>CTAGGGC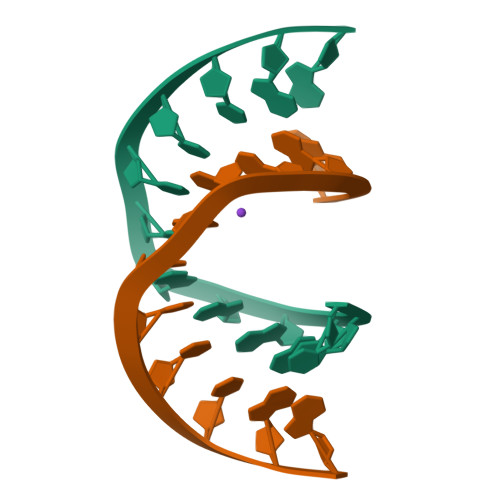CCTAG[2x]>[2x]HTIFQKVSVNGADQGQLKGIRAPANNNPVTDVMSSDIICNAVTMKDSNVLTVPAGAKVGHFWGHEIGG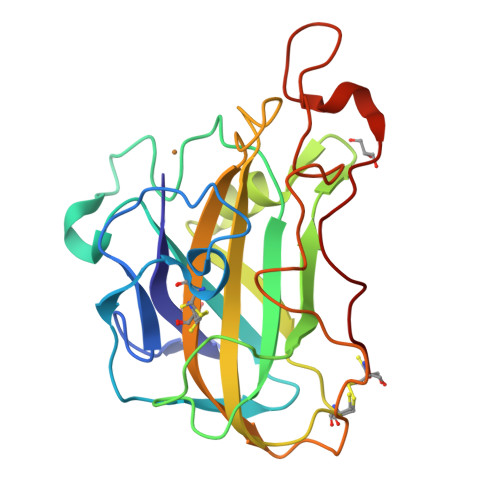AAGPNDADNPIAASHKGPIMVYLAKVDNAATTGTSGLKWFKVAEAGLSNGKWAVDDLIANNGWSYFDMPTCIAPGQYLMRAELIALHNAGSQAGAQFYIGCAQINVTGGGSASPSNTVSFPGAYSASDPGILINIYGGSGKTDNGGKPYQIPGPALFTC> MADTDTQKAD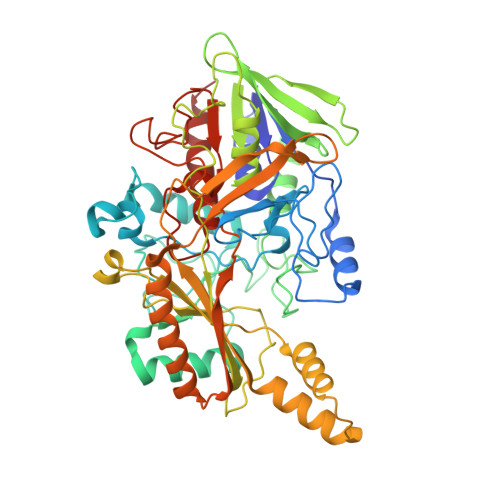VVVVGSGVAGAIVAHQLAMAGKAVILLEAGPRMPRWEIVERFRNQPDKMDFMAPYPSSPWAPHPEYGPPNDYLILKGEHKFNSQYIRAVGGTTWHWAASAWRFIPNDFKMKSVYGVGRDWPIQYDDLEPYYQRAEEELGVWGPGPEEDLYSPRKQPYPMPPLPLSFNEQTIKTALNNYDPKFHVVTEPVARNSRPYDGRPTCCGNNNCMPICPIGAMYNGIVHVEKAERAGAKLIENAVVYKLETGPDKRIVAALYKDKTGAEHRVEGKYFVLAANGIETPKILLMSANRDFPNGVANSSDMVGRNLMDHPGTGVSFYASEKLWPGRGPQEMTSLIGFRDGPFRATEAAKKIHLSNLSRIDQETQKIFKAGKLMKPDELDAQIRDRSARYVQFDCFHEILPQPENRIVPSKTATDAIGIPRPEITYAIDDYVKRGAAHTREVYATAAKVLGGTDVVFNDEFAPNNHITGSTIMGADARDSVVDKDCRTFDHPNLFISSSATMPTVGTVNVTLTIAALALRMSDTLKKEVHHHHHH> XADVAGTSNRDFAGREQRLFNSEQYNYNNSLNGEVSVWVYAYYSDGSVLVINKNSQYKVGISETFKALKEYREGQHNDSYDEYEVNQSIYYPNGGDARKFHSNAKPRAIQIIFSPSVNVRTIKMAKGNAVSVPDEYLQRSHPWEATGIKYRKIKRDGEIVGYSHYFELPHEYNSISLAVSGVHKNPSSYNVGSAHNVM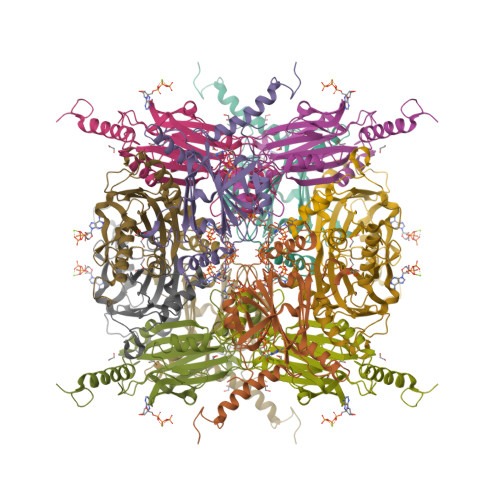DVFQSCDLALRFCNRYWAELELVNHYISPNAYPYLDINNHSYGVALSNRQ>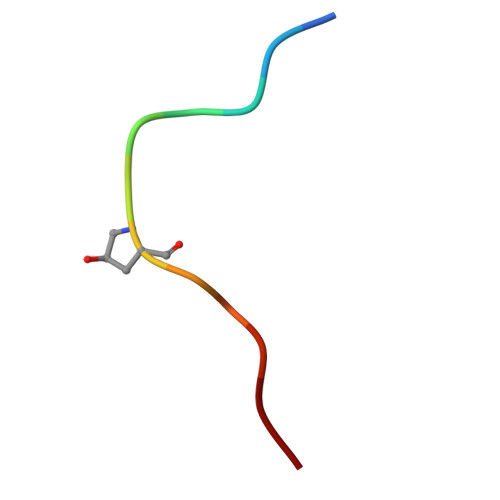 LVPPSGPSMRHN> GAAALKNYYEVHKELFEGVQKWEETWRLFLEFERKASDPNRFTNRGGNLLKEEKQRAKLQKML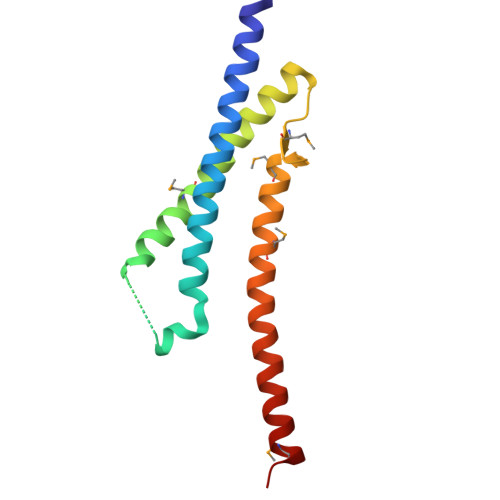PKLEEELKARIELWEQEHSKAFMVNGQKFMEYVAEQWEMHRLEKERAKQERQLKNKKQTETEMLYGS> GSSSGGGSSSSGTSSAFSSYFNNKVGI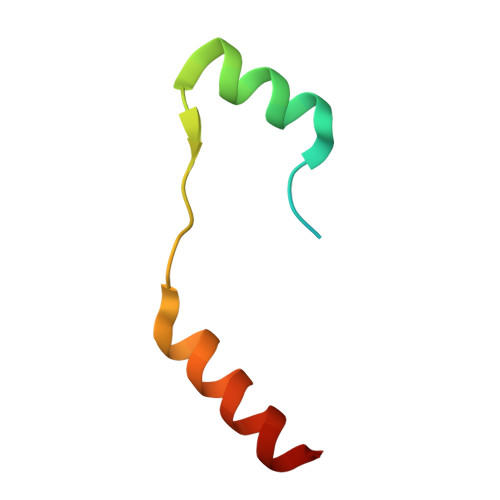PQEHVDHDDFDANQLLNKINE(2S)-2-({9-(1-methylethyl)-6-[(4-pyridin-2-ylbenzyl)amino]-9H-purin-2-yl}amino)butan-1-ol 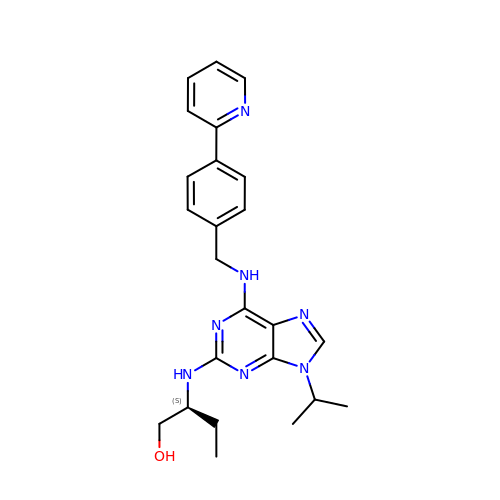| C24 H29 N7 O | HOCBJBNQIQQQGT-IBGZPJMESA-N> AE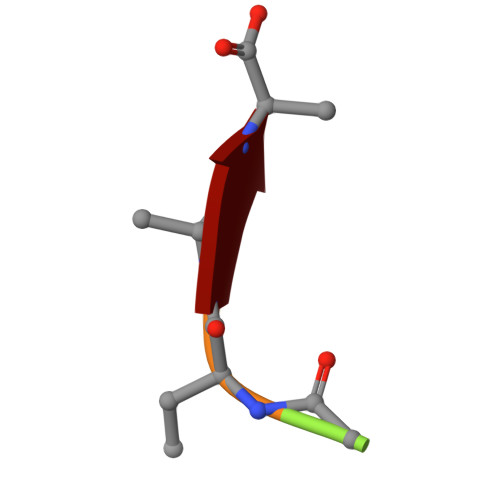KAA>MKLSDIYLELKKGYADSLLYSDLSLLVNIMEYEKDIDVMSIQSLVAGYEKSDTPTITCGIIVYNESKRIKKCLNSVKDDFNEIIVLDSYSTDDTVDIIKCDFPDVEIKYEKWKNDFSYARNKIIEYATSEWIYFIDADNLYSKENKGKIAKVARVLEFFSIDCVVSPYIEEYTGHLYSDTRRMFRLNGKVKFHGKVHEEPMNYNHSLPFNFIVNLKVYHNGYNPSENNIKSKTRRNINLTEEMLRLEPENPKWLFFFGRELHLLDKDEEAIDYLKKS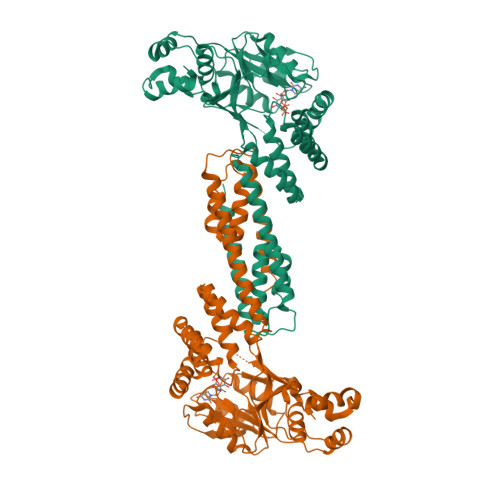INNYKKFNDQRHFIDALVLLCTLLLQRNNYVDLTLYLDILETEYPRCVDVDYFRSAILLVDMQNKLTSLSNMIDEALTDERYSAINTTKDHFKRILISLNIQLENWERVKEISGEIKNDNMKKEIKQYLANSLHNIEHVLKGIEV[2x]> GPGSTEPFGLDRGLELDKVLHCYQMKELFLFVTWKGCSSIDAVPMKY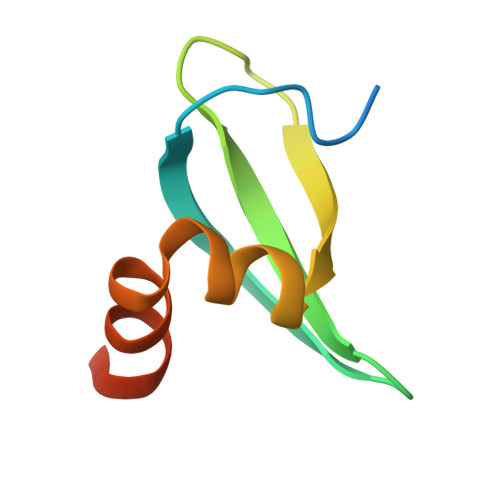IREAYPLQVIEFFQSGSGSGS(hydroxy{(1S)-1-(methylsulfanyl)-2-[5-({4-[(morpholin-4-yl)methyl]phenyl}ethynyl)-1H-benzotriazol-1-yl]ethyl}amino)methanol 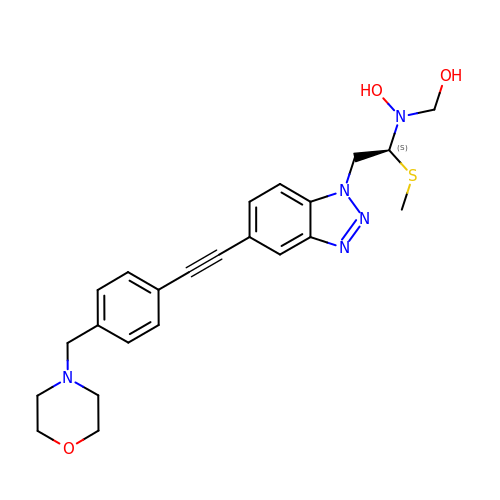| C23 H27 N5 O3 S | AMIXUMKMQGGIQQ-QHCPKHFHSA-N> QGHMSNFLAEQYERDRKAIINCCFSRPDHKTGEPPNNYITHVRIIEDSKFPSSRPPPDSKLENKKKRLLILSAKPNNAKLIQIHKARENSDGSFQIGRTWQLTELVRVEKDLEISEGFILTMSKKYYWETNSAKERTVFIKSLITLYIQTFEGHVPELVNWDLSLFYLDERSYQRAVITNRPGSVSPI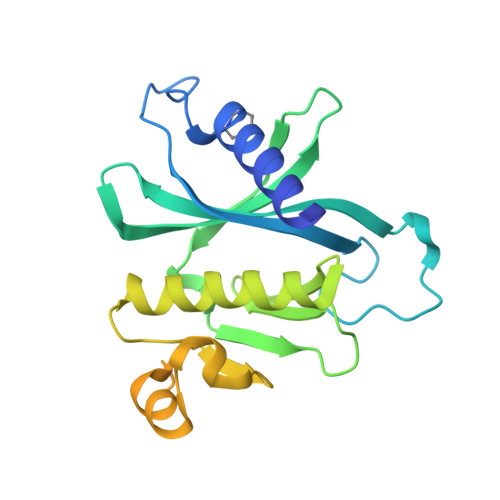KSPTSNFTTNTTQSVGSVPFSAPTERTRRSETESVNPVSTPASVEYHAGMKSLNKAPYSSNS> ATITQDTPINQIFTDTALAEKMKTVLGKTNVTDTVSQTDLDQVTTLQADRLGIKSIDGVEYLNNLTQINFSNNQLTDITPLKNLTKLVDILMNNNQIADITPLANLTNLTGLTLFNNQITDIDPLKNLTNLNRLELSSNTISDISALSGLTSLQQLNFGNQVTDLKPLANLTTLERLDISSNKVSDISVLAKLTNLESLIATNNQISDITPLGILTNLDELSLNGNQLKDIGTLASLTNLTDLDLANNQISNLAPLSGLTKLTELKLGANQISNISPLAGLTALTNLELNENQLEDISPISNLKNLTYLTLYFNNISDISPVSSLTKLQRLFFYNNKVSDVSSLANLTNINWLSAGHNQISDLTPLANLTRITQLGLNDQAWTNAP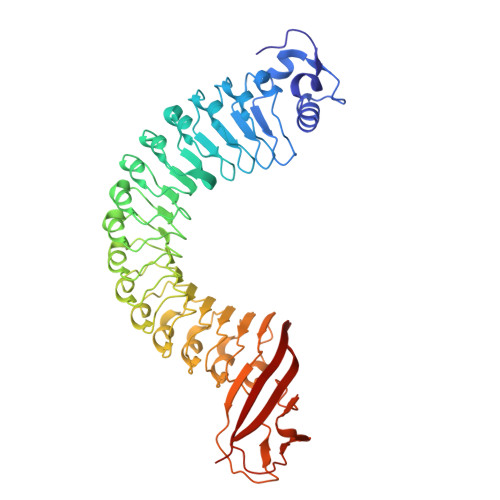VNYKANVSIPNTVKNVTGALIAPATISDGGSYTEPDITWNLPSYTNEVSYTFSQPVTIGKGTTTFSGTVTQPLKA>MDKAKRNIKPFDGEKYAIWKFRIRALLAEQDVLKVVDGLMPNEVDDSWKKAERCAKSTIIEYLSDSFLNFATSDITARQILENLDAVYERKSLASQLALRKRLLSLKLSSEMSLLSHFHIFDELISELLAAGAKIEEMDKISHLLITLPSCYDGIITAIETLSE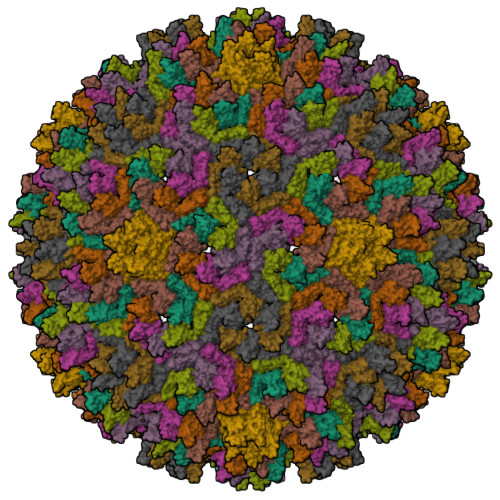ENLTLAFVKNRLLDQEIKIKNDHNDTSKKVMNAIVHNNNNTYKNNLFKNRVTKPKKIFKGNSKYKVKCHHCGREGHIKKDCFHYKRILNNKNKENEKQVQTATSHG[9x]(1R,2S)-1-[(1S)-1,2-dihydroxyethyl]-3-[(2R,3S,4S)-3,4-dihydroxy-2-(hydroxymethyl)tetrahydrothiophenium-1-yl]-2-hydroxypropyl sulfate | C10 H20 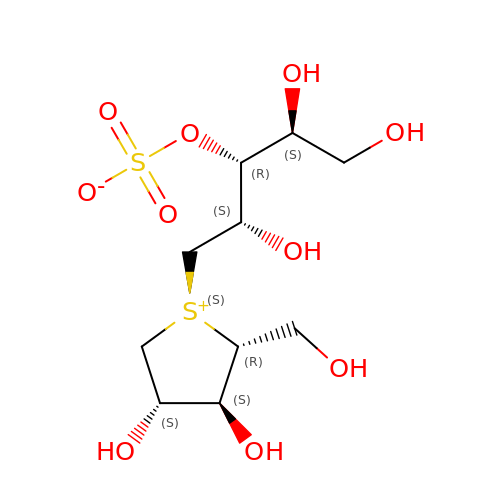O10 S2 | RJAPJYRCCYZVIU-BZCOVLGNSA-N>[2x]MSGLRVYSTSVTGSR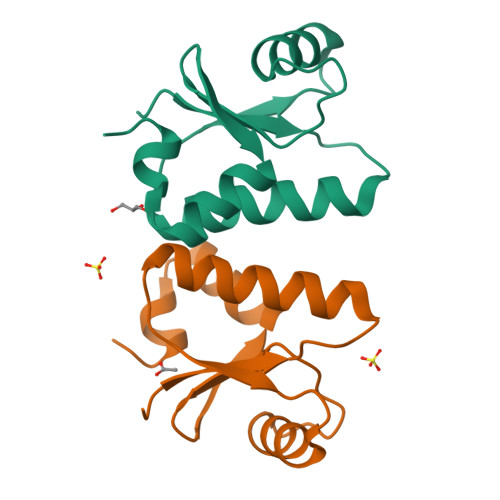EIKSQQSEVTRILDGKRIQYQLVDISQDNALRDEMRTLAGNPKATPPQIVNGNHYCGDYELFVEAVEQDTLQEFLKLA> YKAENGNVKIPKHPKRVVVMADGYYGYFKTLGINVVGAPENVFKNPYYKGKTNGVENIGDGTSVEKVIDLNPDLIIVWTTQGADIKKLE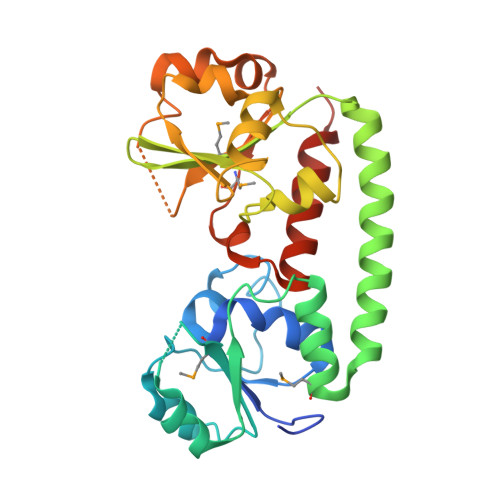KIAPTVAVKYDKLDNIEQLKEFAKMTGTEDKAEKWLAKWDKKVAAAKTKIKKAVGDKTISIMQTNGKDIYVFGKDFGRGGSIIYKDLGLQATKLTKEKAIDQGPGYTSISLEKLPDFAGDYIFAGPWQSGGDDGGVFESSIWKNLNAVKNGHVYKMDPIGFYFTDPISLEGQLEFITESLTKLEHHHHHH>SECNDPFVVALKDKGYSLVAYPKTSIRPLHIYEHTIKNAFKRIWIQSEAQPTSGFIKSLFSDKIHGAIGLSDGQGIDIDLRKTNSLSSAVAAKILESYFQDSAPSFDLAFENSSSVIFHIEEIITTDADEISLRNWLNDNQNELR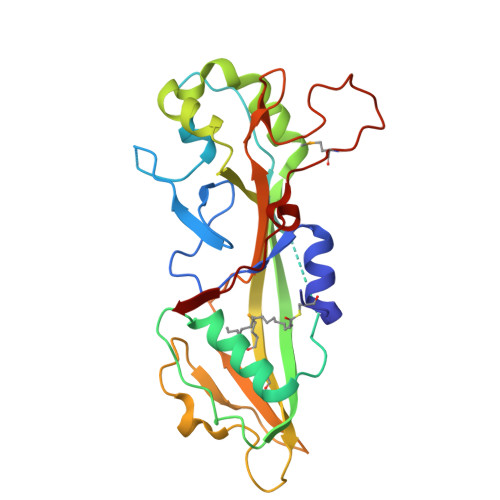EIYKEEIKKGNFFVATSLLRAKKMRMQFERKNKGELGVDVSKIKNLPVDAKLESKIEGSTYDRLVFETPDEGIVFGVKLVRLFFSDNGILTIDKKQDFNRVLGENMALNLFTEIQDAGFIEVT[4x]> QQCNGIYIW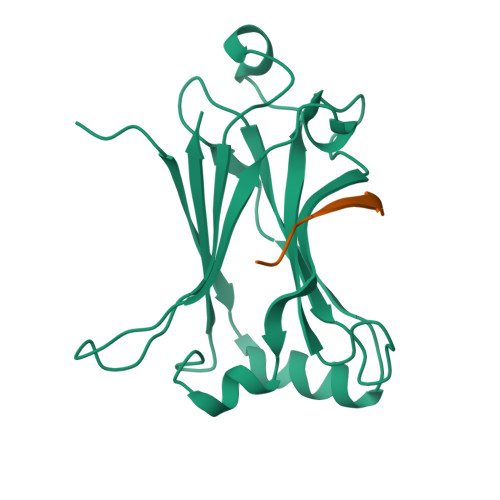KIGNFGMHLKCQEEEKPVVIHSPGFYTGKPGYKLCMRLHLQLPTAQRCANYISLFVHTMQGEYDSHLPWPFQGTIRLTILDQSEAPVRQNHEEIMDAKPELLAFQRPTIPRNPKGFGYVTFMHLEALRQRTFIKDDTLLVRCEVSTRFDLE;> KQEPQEIDF>[6x]MPSLMSFGSCQWIDQGRFSRSLYRNFKTFKLHEMHGLCMPNLLLNPDIHGDRIIFVCCDDLWEHDLKSGSTRKIVSNLGVINNARFFPDGRKIAIRVMRGSSLNTADLYFYNGENGEIKRITYFSGKSTGRRMFTDVAGFDPDGNLIISTDAMQPFSSMTCLYRVENDGINFVPLNLGPATHILFADGRRVIGRNTFELPHWKGYRGGTRGKIWIEVNSGAFKKIVDMSTHVSSPVIVGHRIYFITDIDGFGQIYSTDLDGKDLRKHTSFTDYYPRHLNTDGRRILFSKGGSIYIFNPDTEKIEKIEIGDLESPEDRIISIPSKFAEDFSPLDGDLIAFVSRGQAFIQDVSGTYVLKVPEPLRIRYVRRGGDTKVAFIHGTREGDFLGIYDYRTGKAEKFEENLGNVFAMGVDRNGKFAVVANDRFEIMTVDLETGKPTVIERSREAMITDFTISDNSRFIAYGFPLKHGETDGYVMQAIHVYDMEGRKIFAATTENSHDYA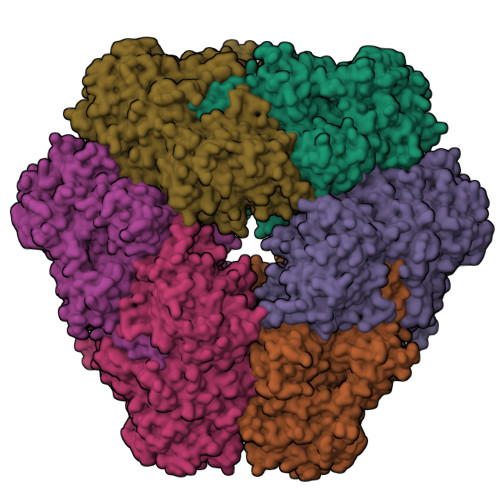PAFDADSKNLYYLSYRSLDPSPDRVVLNFSFEVVSKPFVIPLIPGSPNPTKLVPRSMTSEAGEYDLNDMYKRSSPINVDPGDYRMIIPLESSILIYSVPVHGEFAAYYQGAPEKGVLLKYDVKTRKVTEVKNNLTDLRLSADRKTVMVRKDDGKIYTFPLEKPEDERTVETDKRPLVSSIHEEFLQMYDEAWKLARDNYWNEAVAKEISERIYEKYRNLVPLCKTRYDLSNVIVEMQGEYRTSHSYEMGGTFTDKDPFRSGRIACDFKLDGDHYVVAKAYAGDYSNEGEKSPIFEYGIDPTGYLIEDIDGETVGAGSNIYRVLSEKAGTSARIRLSGKGGDKRDLMIDILDDDRFIRYRSWVEANRRYVHERSKGTIGYIHIPDMGMMGLNEFYRLFINESSYQGLIVDVRFNGGGFVSQLIIEKLMNKRIGYDNPRRGTLSPYPTNSVRGKIIAITNEYAGSDGDIFSFSFKKLGLGKLIGTRTWGGVVGITPKRRLIDGTVLTQPEFAFWFRDAGFGVENYGVDPDVEIEYAPHDYLSGKDPQIDYAIDALIEELRNWNEELPQRPS;>[6x]RVRKX>ADPGGSHHHHHHSRKTYTLTDYLKNTYRLKLYSLRWISDHEYLYKQENNILVFNAEYGNSSVFLENSTFDEFGHSINDYSISPDGQFILLEYNYVKQWRHSYTASYDIYDLNKRQLITEERIPNNTQWVTWSPVGHKLAYVWNNDIYVKIEPNLPSYRITWTGKEDIIYNGITDWVYEEEVFSAYSALWWSPNGTFLAYAQFNDTEVPLIEYSFYSDESLQYPKTVRVPYPKAGAVNPTVKFFVVNTDSLSSVTNATSIQITAPASMLIGDHYLCDVTWATQERISLQWLRRIQNYSVMDICDYDESSGRWNCLVARQHIEMSTTGWVGRFRPSEPHFTLDGNSFYKIISNEEGYRHICYFQIDKKDCTFITKGTWEVIGIEALTSDYLYYISNEYKGMPGGRNLYKIQLSDYTKVTCLSCELNPERCQYYSVSFSKEAKYYQLRCSGPGLPLYTLHSSVNDKGLRVLEDNSALDKMLQNVQMPSKKLDFIILNETKFWYQMILPPHFDKSKKYPLLLDVYAGPCSQKADTVFRLNWATYLASTENIIVASFDGRGSGYQGDKIMHAINRRLGTFEVEDQIEAARQFSKMGFVDNKRIAIWGWSYGGYVTSMVLGSGSGVFKCGIAVAPVSRWEYYDSVYTERYMGLPTPEDNLDHYRNSTVMSRAENFKQVEYLLIHGTADDNVHFQQSAQISKALVDVGVDFQ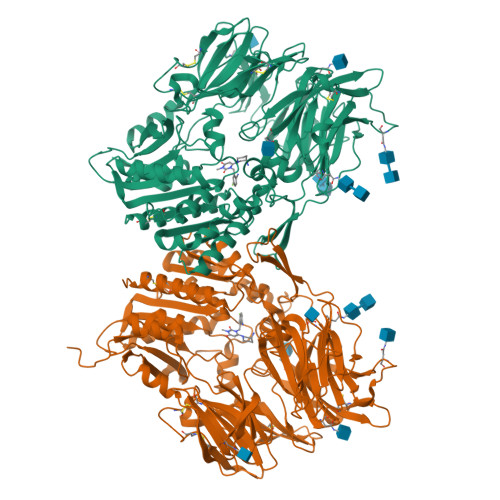AMWYTDEDHGIASSTAHQHIYTHMSHFIKQCFSLP[4x]>AMNLKQALIDNNSIRLGLSADTWQEAVRLAVQPLIDSKAVTSAYYDAIIASTEKYGPYYVLMPGMAMPHAEAGLGVNRNAFALITLTKPVTFSDGKEVSVLLTLAATDPSIHTTVAIPQIVALFELDNAIER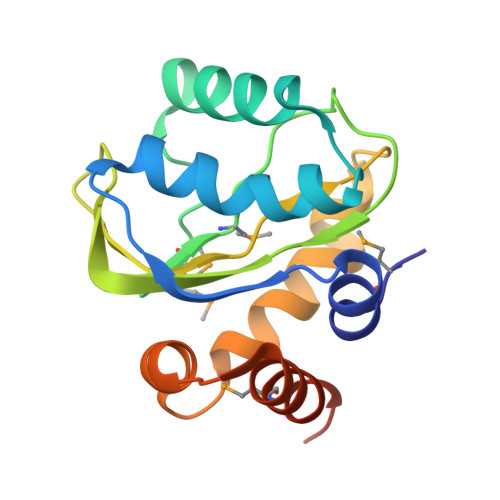LVACQSPKEVLEMVEESKDSPYLEGMDLNA[4x]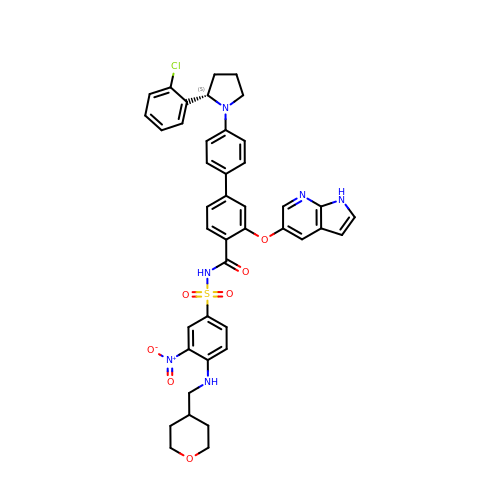4-[4-[(2~{S})-2-(2-chlorophenyl)pyrrolidin-1-yl]phenyl]-~{N}-[3-nitro-4-(oxan-4-ylmethylamino)phenyl]sulfonyl-2-(1~{H}-pyrrolo[2,3-b]pyridin-5-yloxy)benzamide | C42 H39 Cl N6 O7 S | SMXXGDKPPGHBSW-LHEWISCISA-N>[2x]MAILKAQHLAKSYKKRKVVSDVSLQVESGQIVGLLGPNGAGKTTSFYMIVGLVARDEGTITIDDNDISILPMHSRSRMGIGYLPQEASIFRKLSVEDNIMAVLQTREELTHEERQDKLEDLLEEFHIQHIRKSAGMALSGGERRRVEIARALAANPQFILLDQPFAGVDPISVIDIKKIIEHLRDRGLGVLITDHNVRETLDVCEKAYIVSQGRLIAEGTPQDVLNNEQVKQVYLGEQFRL;> MSLSRIVYVLLLFIASWSLYYLLGQEQDSKIQVAPNLELPMFSGENLENISYDEQGIRNYVITSIHLDHYAKSGNTLFKAPILKVYREGTLQEWEITARRGILSKDQVLTLYDDVLAKNLLPDSGFDTLTTSEMSIQLKSRDFWADKPVELRGPQFETHGQAMKGNFADHSAELYNQVQGRYETLTPLVPR;> MIIVRYLIRETIKSQFAIFFVLFLVFLSQKFIRVLADASDGEIPTSMILSIVGLNMPAM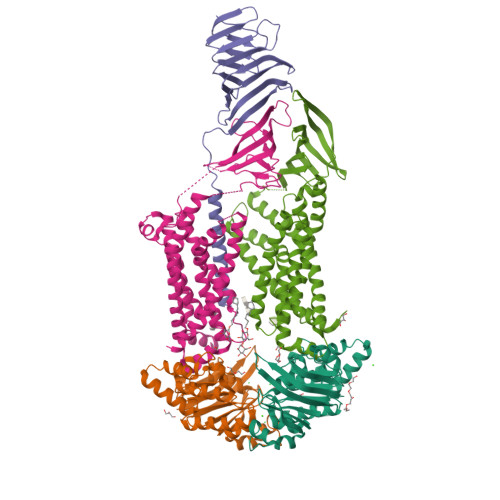GLLMLPLSLYIGILLTFGRLYAESEITVMNATGIGNKFLIRAALYLALITASVAAFNALWLAPWSQDKEAHLMEQFAAENSVDLLQKGHFQRSPDGSSVVFIDNIENRKLYNVFVAQLAPRDSILPSVMFSHSGDVKELSDGRQIITLYDGTRYEGVPTRVDYMITNFDSYDGLIGQREVKSAERDWEALPTLSLLNNADRRAQAELQWRISLVVCIPLLTMLVVPLSAVNPRQGRFAKMGPAILIYLTYFLALSATKSAIEDGSLPVIIGLWPINAALLLAALMVNTLDSIPVRRFKDRWKQRKVA;> MFKILDWYIGRTIVATTALVLVTFVGLSGIIKYVEQLRKVGEGSYDLLQALLFVVLSIPRDVEMFFPMAALLGALIGLGALASSSELVVMQAAGFSKLDIGLSVLKTAIPLMIIVTLLGEWGAPQAQKMARDMRAFATSGGAIMSVRTGVWARDANDFIFIAKVENEHLYGLNLWRFDENKKLSTVIFSEQVDYVANNEWLMKDAVLTRLVNDIEISKESLPEYRWRTSLAPDKLAVVTVKPEELSLTGLSDYVHYLKASEQDSSRYELALWRKVTQPISIAVMMLMALSFIFGPLRSVTMGARILSGVIAGFSFYISSEFFGPLSLVYGLPPLFGALAPSLVFLAIALGLLGRKL> MNPEKMNNAKVANMPSTEGLPSLPQ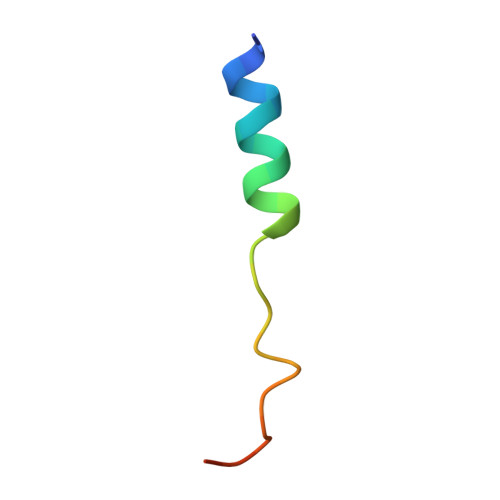GE> VNYWV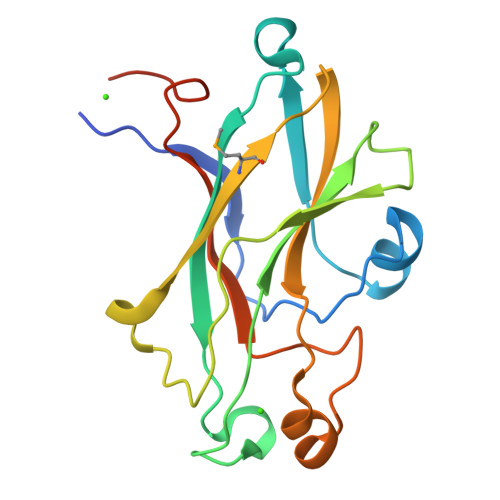SDEEIRVFKEYSARAKYAQNEGRTALEANNVPFFDIDVPPELDGVPFSLKARVRHKSKGVDGLGDYTSISVKPAFYITEGDETTDTLIKYTSYGSTGSHSGYDFDDNTLDVMVTLSAGVHRVFPVETELDYDAVQEVQHDWYDESFTTFIEVYSDDPLLTVKGYAQILMERT> APAWL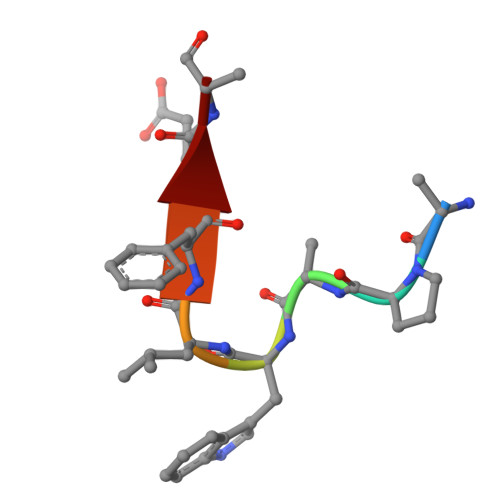FEA(2~{R},3~{S},4~{S},5~{S})-5-fluoranyl-2-(hydroxymethyl)oxane-3,4-diol | C6 H11 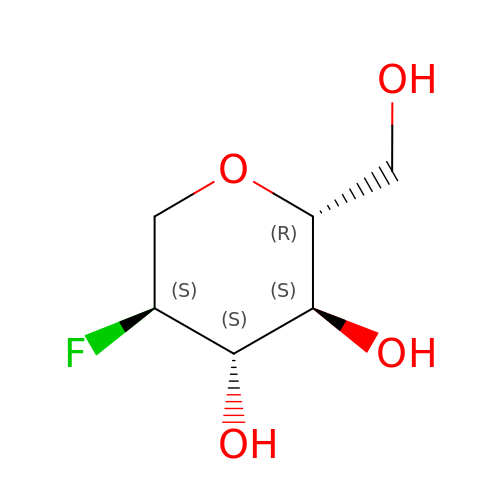F O4 | JEWFVWVAXVTBRL-SLPGGIOYSA-N> GTGDAAPGASKLRAVLEKLKLSRDDISTAAGMVKGVVDHLLLRLKCDSAFRGVGLLNTGSYYEHVKISAPNEFDVMFKLEVPRIQLEEYSNTRAYYFVKFKRNPKENPLSQFLEGEILSASKMLSKFRKIIKEEINDIKDTDVIMKRKRGGSPAVTLLISEKISVDITLALESKSSWPASTQEGLRIQNWLSAKVRKQLRLKPFYLVPKHAKEGNGFQEETWRLSFSHIEKEILNNHGKSKTCCENKEEKCCRKDCLKLMKYLLEQLKERFKDKKHLDKFSSYHVKTAFFHVCTQNPQDSQWDRKDLGLCFDNCVTYFLQCLRTEKLENYFIPEFNLFSSNLIDKRSKEFLTKQIEYERNNEFPVFDEF

Cyclic GMP-AMP (cGAMP) synthase (cGAS) is essential for the host defense against cytosolic double-stranded (ds)DNA arising from various maladies (e.g., pathogen invasion, ionizing irradiation, and genotoxic chemicals). Upon directly binding to and dimerizing on dsDNA, cGAS cyclizes ATP and GTP into 2′−5′/3′−5′-linked cGAMP, a unique metazoan second messenger for initiating type-I interferon (IFN-I)-mediated inflammatory responses. cGAS is central to antitumor immunity, host defense against an array of pathogens, and regulating autoimmunity. Here, we resolve these numerous fundamental mechanistic questions in innate immunology and present a unifying catalytic mechanism of cGAS. Finally, we reveal how mouse cGAS achieves more stringent substrate selectivity and higher catalytic efficiency than the human enzyme. Together, we set forth a unifying catalytic mechanism of cGAS in which dsDNA-binding pre-organizes the active site into a rigid yet adaptable lock for two sets of keys (substrates and intermediate) necessary to specifically synthesize 2′−5/3′−5′-cGAMP.

To further examine these discrepancies, we crystallized and solved the structure of the catalytic domain of human cGAS (hcGAScat). We noted that, unlike the mouse enzyme, the three β-sheets do not move upon dsDNA binding, while the catalytic residues assume different rotamer conformations. However, the activation loop in our structure was mostly disordered (thus not modeled in Fig. 1D and Supplementary Fig. 1A). Comparing the B-factors of hcGAScat structures with or without bound dsDNA revealed that, while the C-lobe remains steady (likely via dimerization/crystal contact), dsDNA drastically stabilizes the N-lobe containing the activation loop and the catalytic residues. Together, our observations suggest that, instead of being fixed into a specific autoinhibited conformation, the active site of resting cGAS assumes an array of inactive states and its activation entails a dsDNA-dependent disorder-to-order transition. D An overlay of dsDNA-free and dsDNA-bound WT-hcGAScat structures.> VESSTDGQVVPQEVLNLPLEKAHEEADDYLDHLLD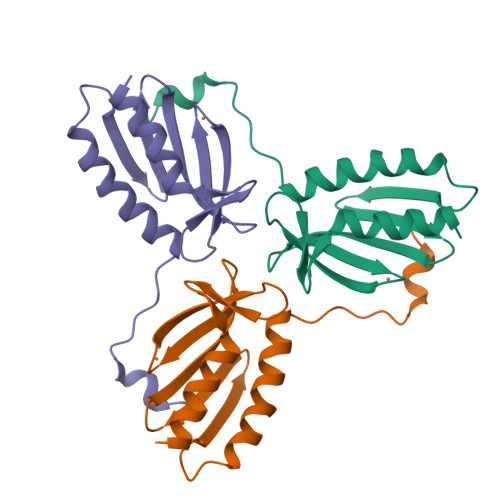SLEELSEAHPDCIPDVELSHGVMTLEIPAFGTYVINKQPPNKQIWLASPLSGPNRFDLLNGEWVSLRNGTKLTDILTEEVEKAISKSQ>[2x]GFDGAISDDSLRQVGESEVWVPFIHSKGNAGIGKTGGKRVDFEGLAGGIFDDERNGVHTSGSKHFQDNFYSFVQVANQDV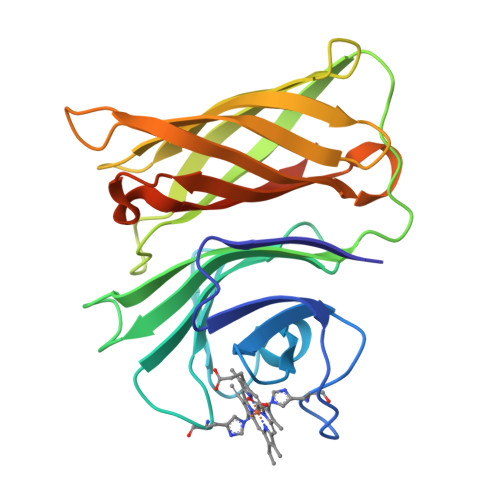WFGEWYEGKKDSEFNNRTVYYVGNDAGTTVPTSGKATYNITGINKFSGANKLSGTFNADFGAKTLDGSINNSNLTVSVDATINAATAAFNGTAQAVQNGTTTNGASQGHFFGANAAGLAGIATFTNNSDLDTAFGGEKKELALVPRGSHHHHHH Spermidine synthase (SpdS; putrescine aminopropyltransferase) catalyzes the transfer of the aminopropyl moiety from decarboxylated S-adenosylmethionine to putrescine, leading to the formation of spermidine and 5′-methylthio­adenosine (MTA). In this work, X-ray crystallography was used to examine ligand complexes of SpdS from the malaria parasite Plasmodium falciparum (PfSpdS). The active site of SpdS is located between the domains and consists of two interconnected clefts for binding dcAdoMet and putrescine. A conserved flexible structural element called the gatekeeper loop covers the active site of the enzyme.

The complexes with the aniline compounds and BIPA revealed a new mode of ligand binding to PfSpdS. The aminomethyl N atom is positioned at a hydrogen-bonding distance from the carboxylate O atoms of Asp196, the backbone carbonyl O atom of Ser197 and a water molecule. However, in this case the distances to the hydroxyl O atom of Tyr102 are longer (∼4 Å) than the respective distance observed for the putrescine N atom (3.2 Å). The aromatic ring can also engage in a π-stacking interaction with Tyr264, with a ring centre-to-centre distance of 4.0 Å. The binding mode of MTA was essentially identical to those found in the other structures. The results establish experimentally that the putrescine-binding site may accommodate small aromatic compounds and not only aliphatic amines, a finding which, together with the other results, may lead to new approaches for the design of SpdS inhibitors.

>KKWFSEFSIMWPGQAFSLKIKKILYETKSKYQNVLVFESTTYGKVLVLDGVIQLTEKDEFAYHEMMTHVPMTVSKEPKNVLVVGGGDGGIIRELCKYKSVENIDICEIDETVIEVSKIYFKNISCGYEDKRVNVFIEDASKFLENVTNTYDVIIVDSSDPIGPAETLFNQNFYEKIYNALKPNGYCVAQCESLWIHVGTIKNMIGYAKKLFKKVEYANISIPTYPCGCIGILCCSKTDTGLTKPNKKLESKEFADLKYYNYENHSAAFKLPAFLLKEIENI[3x]> DLPMPMRFRHLKKTSKEAVGVYRSPIHGRGLFCKRNIDAGEMVIEYAGIVIRSILTDKREKYYDSKGIGSSYMFRIDDSEVVDATMHGNAARFINHSCEPNCYSRVINID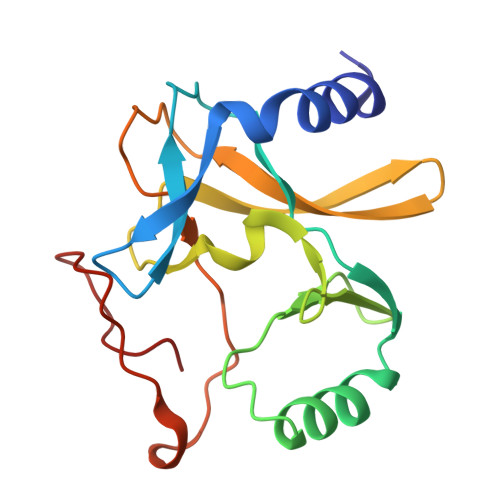GQKHIVIFAMRKIYRGEELTYDYKFPIEDASNKLPCNCGAKKCRKFLN5-[(1E)-2-(2-methoxyphenyl)-4-methylpent-1-en-1-yl]furo[2,3-d]pyrimidine-2,4-diamine | C19 H22 N4 O2 | 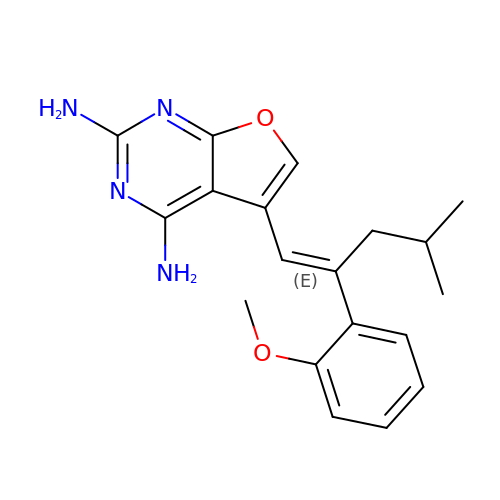GSEWOBPWXZKJLQ-FMIVXFBMSA-N> GHMASDTFTLNTPAYA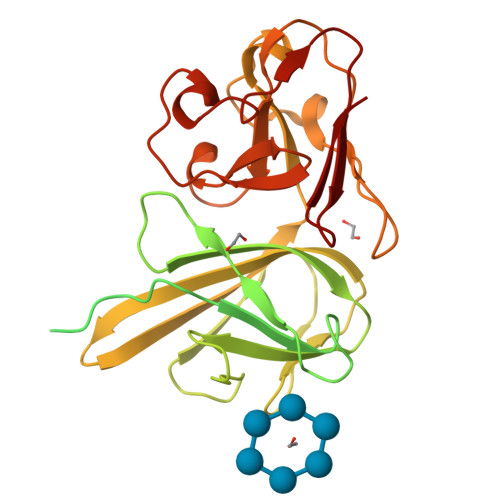ANNVYDLKNAQTVELTCSQPDYGFPAATTYTVQASFEQDFIEATDESKANYTVLESTSPTAKINVDASELNNALLDLWTAVNGEQAELPTEPVAVYIRLKANITSSGKGVCFSNVIELPNVLISKSTSSLTPPKTMFIVGSMLDTDWKVWKPMAGVYGMDGQFYSMIYFDANSEFKFGTKENEYIGINDNRVTVTDKAGAGVSGSDNFVVENAGWYLFYVKAAVKGDDYQFTITFYPAEVYLFGNTTGGSWAFNDEWKFTVPATKDGNFVSPAMTASGEVRMCFKTDLDWWRTEFTLHDGEIFYRDFNLIDSWTEKGDGYSIQGSAGNVIHLNFTAGTGEKK(1-ethyl-1H-benzoimidazol-2-yl)-furan-2-ylmethyl-aminee | C14 H15 N3 O | 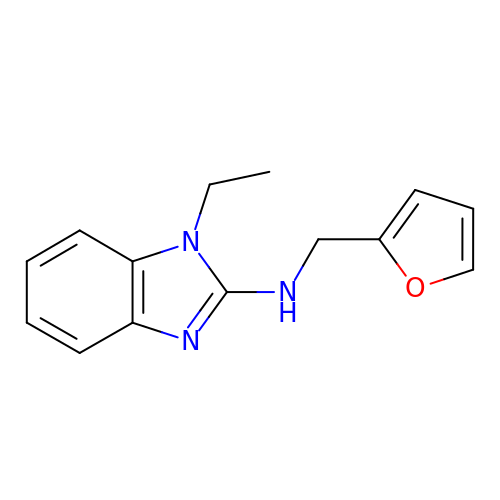XVKUMXLSEKBYCF-UHFFFAOYSA-N>[2x]MGSSHHHHHHSSGLVPRGSGDYDYLIKLLALGDSGVGKTTFLYRYTDNKFNPKFITTVGIDFR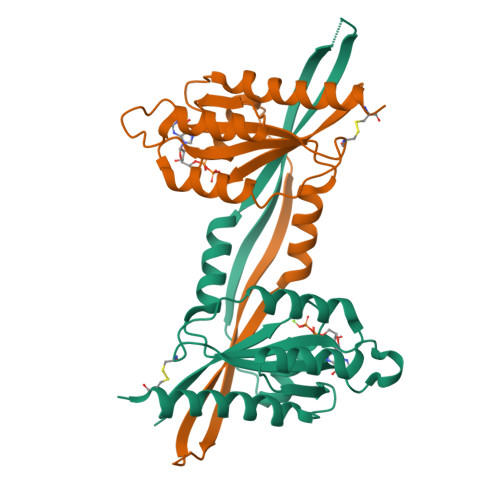EKRVVYNAQGPNGSSGKAFKVHLQLWDTAGQERFRSLTTAFFRDAMGFLLMFDLTSQQSFLNVRNWMSQLQANAYCENPDIVLIGNKADLPDQREVNERQARELADKYGIPYFETSAATGQNVEKAVETLLDLIMKRMEQCVEKTQIPDTVNGG> PISPIETVPVKLKPGMDGPKVKQWPLTEEKIKALVEICTEMEKEGKISKIGPENPYNTPVFAIKKKNSTRWRKLVDFRELNKRTQDFWEVQLGIPHPAGLKKKKSVTVLDVGDAYFSVPLDEDFRKYTAFTIPSINNETPGIRYQYNVLPQGWKGSPAIFQSSMTKILEPFRKQNPDIVIYQYMDDLYVGSDLEIGQHRTKIEELRQHLLRWGLFTPDQKHQKEPPFLWMGYELHPDKWTVQPIVLPEKDSWTVNDI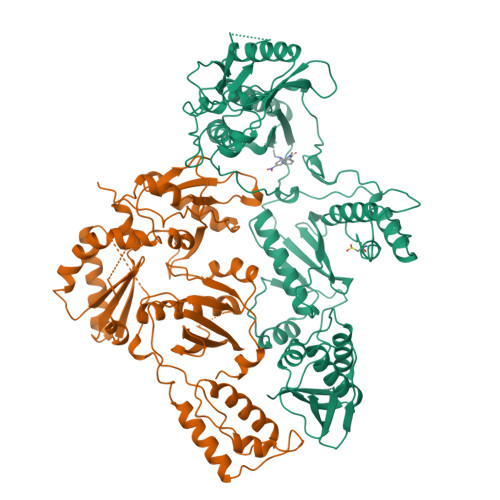QKLVGKLNWASQIYPGIKVRQLCKLLRGTKALTEVIPLTEEAELELAENREILKEPVHGVYYDPSKDLIAEIQKQGQGQWTYQIYQEPFKNLKTGKYARMRGAHTNDVKQLTEAVQKITTESIVIWGKTPKFKLPIQKETWETWWTEYWQATWIPEWEFVNTPPLVKLWYQLEKEPIVGAETFYVDGAANRETKLGKAGYVTNRGRQKVVTLTDTTNQKTELQAIYLALQDSGLEVNIVTDSQYALGIIQAQPDQSESELVNQIIEQLIKKEKVYLAWVPAHKGIGGNEQVDKLVSAGIRKVL;> PISPIETVPVKLKPGMDGPKVKQWPLTEEKIKALVEICTEMEKEGKISKIGPENPYNTPVFAIKKKNSTRWRKLVDFRELNKRTQDFWEVQLGIPHPAGLKKKKSVTVLDVGDAYFSVPLDEDFRKYTAFTIPSINNETPGIRYQYNVLPQGWKGSPAIFQSSMTKILEPFRKQNPDIVIYQYMDDLYVGSDLEIGQHRTKIEELRQHLLRWGLTTPDKKHQKEPPFLWMGYELHPDKWTVQPIVLPEKDSWTVNDIQKLVGKLNWASQIYPGIKVRQLCKLLRGTKALTEVIPLTEEAELELAENREILKEPVHGVYYDPSKDLIAEIQKQGQGQWTYQIYQEPFKNLKTGKYARMRGAHTNDVKQLTEAVQKITTESIVIWGKTPKFKLPIQKETWETWWTEYWQATWIPEWEFVNTPPLVKLWYQLEKEPIVGAETF>MSSVSLQDFDAERIGLFHEDIKRKFDELKSKNLKLDLTRGKPSSEQLDFADELLALPGKGDFKAADGTDVRNYGGLDGIVDIRQIWADLLGVPVEQVLAGDASSLNIMFDVISWSYIFGNNDSVQPWSKEETVKWICPVPGYDRHFSITERFGFEMISVPMNEDGPDMDAVEELVKNPQVKGMWVVPVFSNPTGFTVTEDVAKRLSAMETAAPDFRVVWDNAYAVHTLTDEFPEVIDIVGLGEAAGNPNRFWAFTSTSKITLAGAGVSFFLTSAENRKWYTGHAGIRGIGPNKVNQLAHARYFGDAEGVRAVMRKHAASLAPKFNKVLEILDSRLAEYGVAQWTVPAGGYFISLDVVPGTASRVAELAKE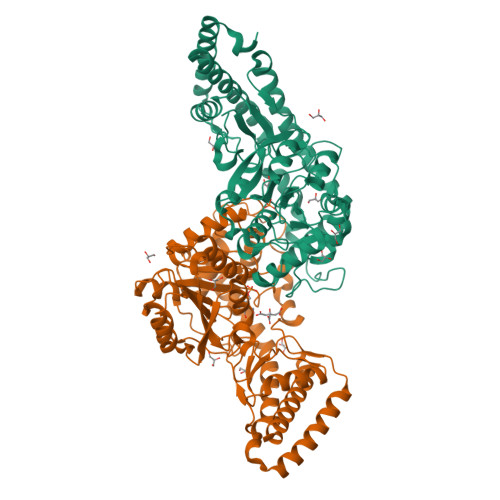AGIALTGAGSSYPLRQDPENKNLRLAPSLPPVEELEVAMDGVATCVLLAAAEHYANLEHHHHHH[2x]> MVSRLSTGILDFDKLIQGGIPQGFFIALTGEPGTGKTIFSLHFIAKGLRDGDPCIYVTTEESRDSIIRQAKQFNWDFEEYIE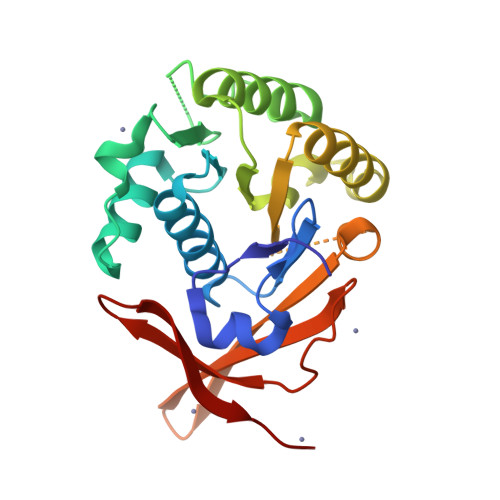KKLIIIDALMKEKEDQWSLVNLTPEELVNKVIEAKQKLGYGKARLVIDSVSALFLDKPAMARKISYYLKRVLNKWNFTIYATSQYAITTSQAFGFGVEHVADGIIRFRRMIRNGELHRYILIEKMRQTDHDKHVWEIDIVNGKGIVLKGRLEE> MKNVGFIGWRGMVGSVLMDRMSQENDFENLNPVFFTTSQAGQKAPVFGGKDAGDLKSAFDIEELKKLDIIVTCQGGDYTNEVYPKLKATGWDGYWVDAASALRMKDDAIIVLDPVNQHVISEGLKKGIKTFVGGNCTVSLMLMAIGGLFEKDLVEWISVATYQAASGAGAKNMRELLSQMGLLEQAVSSELKDPASSILDIERKVTAKMRADNFPTDNFGAALGGSLIPWIDKLLPETGQTKEEWRGYAETNKILGLSDNPIPVDGLCVRIGALRCHSQAFTIKLKKDLPLEEIEQI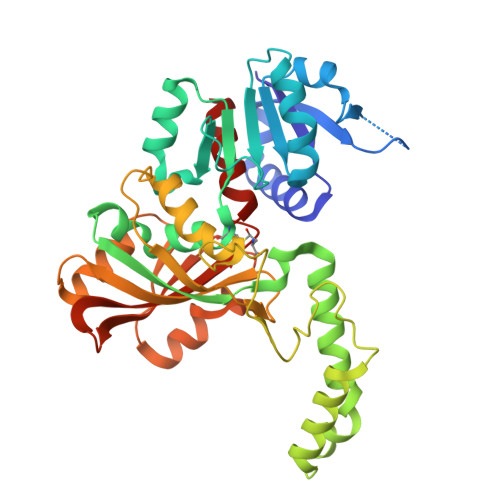IASHNEWVKVIPNDKEITLRELTPAKVTGTLSVPVGRLRKLAMGPEYLAAFTVGDQLLWGAAEPVRRILKQLVA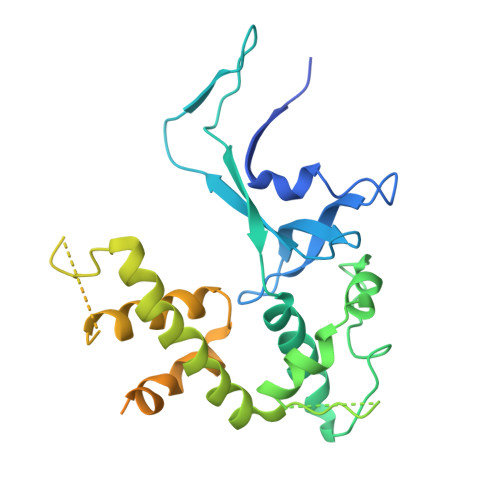> MAAGVDCGDGVGARQHVFLVSEYLKDASKKMKNGLMFVKLVNPCSGEGAIYLFNMCLQQLFEVKVFKEKHHSWFINQSVQSGGLLHFATPVDPLFLLLHYLIKADKEGKFQPLDQVVVDNVFPNCILLLKLPGLEKLLHHVTEEKGNPEIDNKKYYKYSKEKTLKWLEKKVNQTVAALKTNNVNVSSRVQSTAFFSGDQASTDKEEDYIRYAHGLISDYIPKELSDDLSKYLKLPEPSASLPNPPSKKIKLSDEPVEAKEDYTKFNTKDLKTEKKNSKMTAAQKALAKVDKSGMKSIDTFFGVKNKKKIGKV>[6x]MTQMSDEQFRIFIETIKSLGPIKEEPPSKGSFSNCTVRF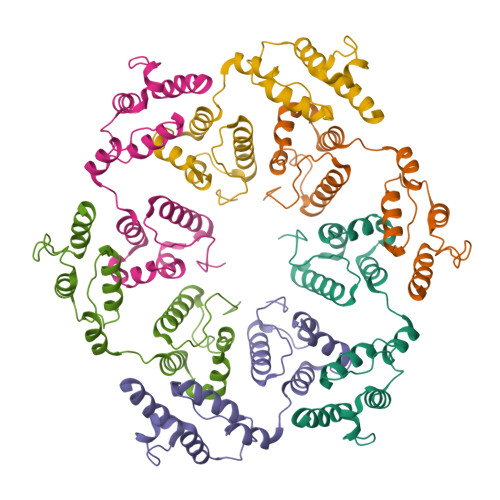SGQRDHDAVDEFINAVETYKEVEGISDKDALKGLPLLFKSIAVVWWKGVRRDAKTWSDALQLLRDHFSPTKPSYQIYMEIFETKQSYDEVIDSFICKQRALLAKLPEGRHDEETELDFIYGLMQPKYRESIPRHEVKTFRELLDRGRTVERTRH>GSMSQAIPS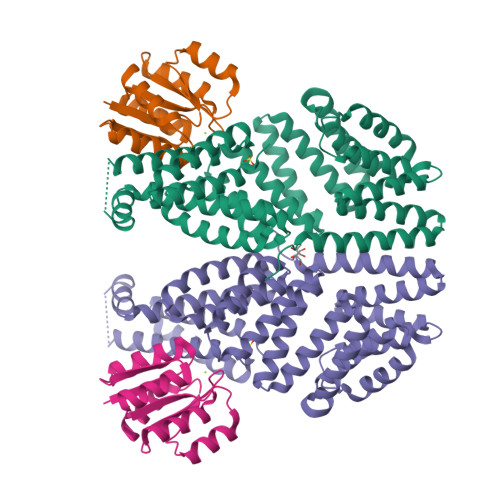SRVGVKINEWYKMIRQFSVPDAEILKAEVEQDIQQMEEDQDLLIYYSLMCFRHQLMLDYLEPGKTYGNRPTVTELLETIETPQKKLTGLLKYYSLFFRGMYEFDQKEYVEAIGYYREAEKELPFVSDDIEKAEFHFKVAEAYYHMKQTHVSMYHILQALDIYQNHPLYSIRTIQSLFVIAGNYDDFKHYDKALPHLEAALELAMDIQNDRFIAISLLNIANSYDRSGDDQMAVEHFQKAAKVSREKVPDLLPKVLFGLSWTLCKAGQTQKAFQFIEEGLDHITARSHKFYKELFLFLQAVYKETVDERKIHDLLSYFEKKNLHAYIEACARSAAAVFESSCHFEQAAAFYRKVLKAQEDILKGECLYAY[2x];>GSMMNEKILIVDDQYGIRILLNEVFNKEGYQTFQAANGLQALDIVTKERPDLVLLDMKIPGMDGIEILKRMKVIDENIRVIIMTAYGELDMIQESKELGALTHFAKPFDIDEIRDAVKKYLPLKSN[2x]>[3x]SNAM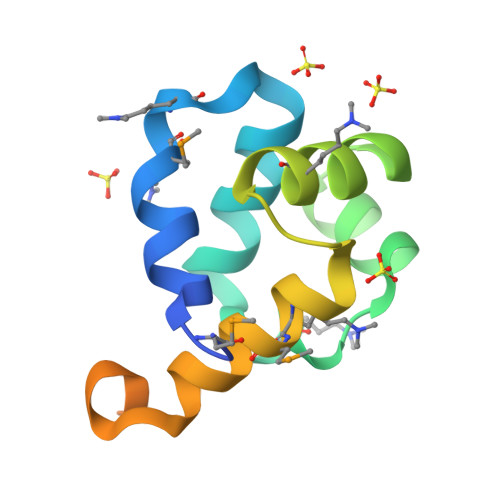ATGGLAIIQSMKHKLPPSERKLADYILAHPHKAIESTVNEISALANSSDAAVIRLCKSLGLKGFQDLKMRVAGDLAKPTFQGYRDIVPHEPLPSISEKTAGNAIQAI>[8x]MSLDWTCKHHADLTLKELYALLQLRTEVFVVEQKCPYQEVDGLDLVGDTHHLMAWRDGQLLAYLRLLDPVRHEGQVVIGRVVSSSAARGQGLGHQLMERALQ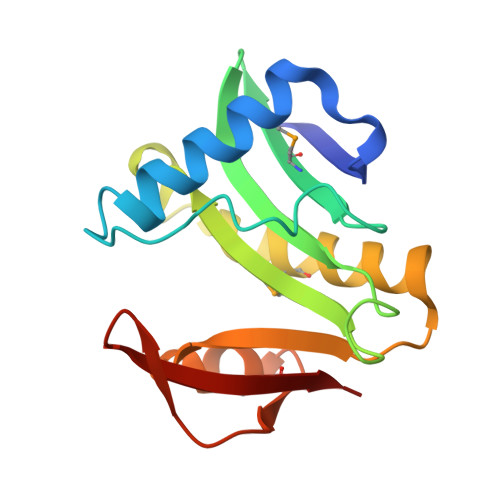AAERLWLDTPVYLSAQAHLQAYYGRYGFVAVTEVYLEDDIPHIGMRRA> QEVEFDIPPQALGSALQEFGRQADIQVLYRPEEVRNKRSSAIKGKLEPNQAITELLRGTGASVDFQGNAITISVAEAADSSVDLGATMITSNQLGTITEDSGSYTPGTIATATRLVLTPRETPQSITVVTRQNMDDFGLNNIDDVMRHTPGITVSAYDTDRNNYYARGFSINNFQYDGIPSTARNVGYSAGNTLSDMAIYDRVEVLKGATGLLTGAGSLGATINLIRKKPTHEFKGHVELGAGSWDNYRSELDVSGPLTESGNVRGRAVAAYQDKHSFMDHYERKTSVYYGILEFDLNPDTMLTVGADYQDNDPKGSGWSGSFPLFDSQGNRNDVSRSFNNGAKWSSWEQYTRTVFANLEHNFANGWVGKVQLDHKINGYHAPLGAIMGDWPAPDNSAKIVAQKYTGETKSNSLDIYLTGPFQFLGREHELVVGTSASFSHWEGKSYWNLRNYDNTTDDFINWDGDIGKPDWGTPSQYIDDKTRQLGSYMTARFNVTDDLNLFLGGRVVDYRVTGLNPTIRESGRFIPYVGAVYDLNDTYSVYASYTDIFMPQDSWYRDSSNKLLEPDEGQNYEIGIKGEYLDGRLNTSLAYFEIHEENRAEEDALYNSKP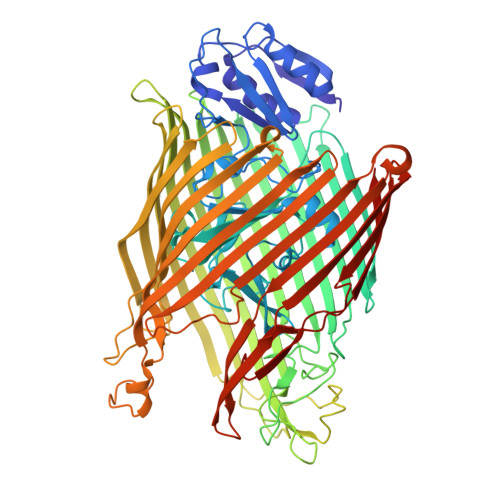TNPAITYAYKGIKAKTKGYEAEISGELAPGWQVQAGYTHKIIRDDSGKKVSTWEPQDQLSLYTSYKFKGALDKLTVGGGARWQGKSWQMVYNNPRSRWEKFSQEDYWLVDLMARYQITDKLSASVNVNNVFDKTYYTNIGFYTSASYGDPRNLMFSTRWDF(2,5-dimethylpyrazol-3-yl)methylcarbamic acid | C7 H11 N3 O2 | 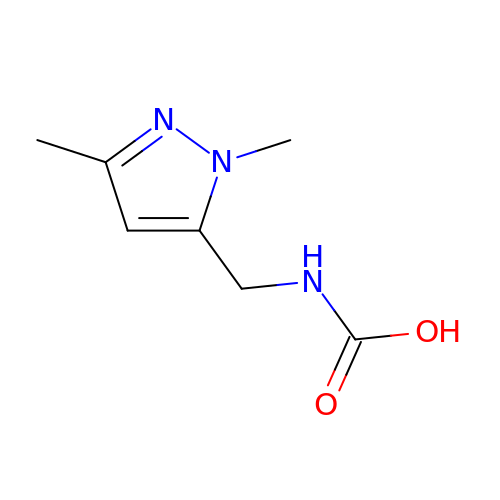GIQHHEQBVBVTAS-UHFFFAOYSA-N> TFAYKIDGNEVIFTLWAPYQKSVKLKVLEKGLYEMERDEKGYFTITLNNVKVRDRYKYVLDDASEIPDPASRYQPEGVHGPSQIIQESKEFNNETFLKKEDLIIYEIHVGTFTPEGTFEGVIRKLDYLKDLGITAIEIMPIAQFPGKRDWGYDGVYLYAVQNSYGGPEGFRKLVDEAHKKGLGVILDVVYNHVGPEGNYMVKLGPYFSQKYKTPWGLTFNFDDAESDEVRKFILENVEYWIKEYNVDGFRLSAVHAIIDTSPKHILEEIADVVHKYN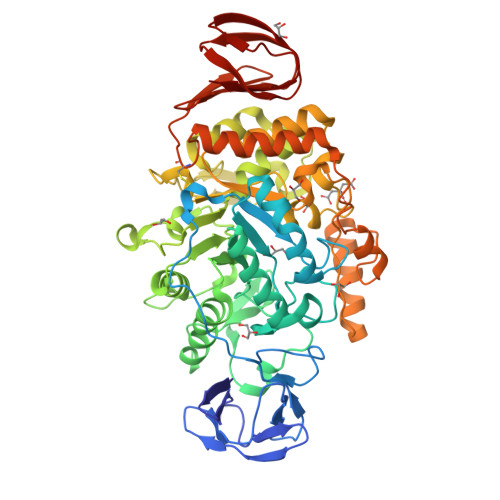RIVIAESDLNDPRVVNPKEKCGYNIDAQWVDDFHHSIHAYLTGERQGYYTDFGNLDDIVKSYKDVFVYDGKYSNFRRKTHGEPVGELDGCNFVVYIQNHDQVGNRGKGERIIKLVDRESYKIAAALYLLSPYIPMIFMGEEYGEENPFYFFSDFSDSKLIQGVREGRKKENGQDTDPQDESTFNASKLSWKIDEEIFSFYKILIKMRKELSIACDRRVNVVNGENWLIIKGREYFSLYVFSKSSIEVKYSGTLLLSSNNSFPQHIEEGKYEFDKGFALYKL The Nucleoside diphosphate linked to another moiety, X (Nudix) superfamily of proteins constitute pyrophosphohydrolases of substrates that include (d)NTPs, nucleotide sugars, capped (m7Gppp and Gppp) RNAs and dinucleotide coenzymes including NAD, FAD, dephosphoCoA (dpCoA) and their derivatives. Among the Nudix proteins, Nudt16 is the most promiscuous. Similar to DXO, it can hydrolyze RNAs harboring an m7G cap, unmethylated cap, NAD cap, dpCoA cap and FAD cap on the 5′end. To understand the molecular mechanism for the recognition of FAD-capped RNA by Nudt16, we determined the crystal structure of human Nudt16 in complex with FAD at 2.7 Å resolution and the structure of free human Nudt16 at 2.3 Å resolution.

FAD is bound in the active site of Nudt16. An entire FAD molecule is observed in the active site of one monomer, while only AMP is observed in the active site of the other monomer, likely due to hydrolysis during crystallization and consistent with the deFADding activity of Nudt16. In this binding mode, the 3′ hydroxyl group of the ribose is exposed to the solvent, and the first few nucleotides of the RNA body could have interactions with the loop containing residues 101–106. The adenine base of FAD is π-stacked with the side chain of His24 on one face and positioned against Ile164 on the other. The N1 atom of adenine is hydrogen-bonded to the side chain of Gln170, and the N6 atom is located near the main-chain amide nitrogen of Phe57. The α phosphate is coordinated to a Mn2+ ion in the active site and has hydrogen-bonding interactions with His24. The β phosphate is involved in ionic interactions with the side chain of Arg50. The flavin ring is π-stacked against the side chain of Phe36, from the other monomer of the dimer, while the other face of the flavin ring is exposed to solvent. The side chain of Arg38, also from the other monomer, has hydrogen-bonding interaction with the N5 atom of the flavin ring. The AMP portion of FAD is bound at a location generally similar to that of equivalent moiety in other compounds, such as the m7GpppA cap, inosine monophosphate (IMP) and ADP-ribose, suggesting that the deFADding activity shares the same catalytic mechanism as these other reactions.

>[2x]MAGARRLELGEALALGSGWRHACHALLYAPDPGMLFGRIPLRYAILMQMRFDGRLGFPGGFVDTQDRSLEDGLNRELREELGEAAAAFRVERTDYRSSHVGSGPRVVAHFYAKRLTLEELLAVEAGATRAKDHGLEVLGLVRVPLYTLRDGVGGLPTFLENSFIGSAREQLLEALQDLGLLQSG>GGTGTGTGTGTGG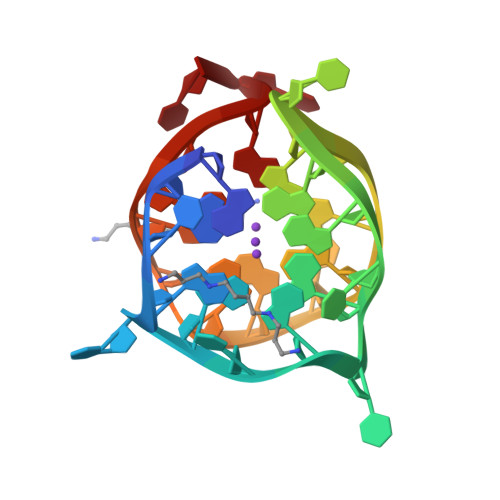TGTGGTGGTGGTGTT[2x]>[2x]QYVRIKNWGSGEILHDTLHHKATSDFTCKSKSCLGSIMNPKSLTRGPRDKPTPLEELLPHAIEFINQYYGSFKEAKIEEHLARLEAVTKEIETTGTYQLTLDELIFATKMAWRNAPRCIGRIQWSNLQVFDARNCSTAQEMFQHICRHILYATNNGNIRSAITVFPQRSDGKHDFRLWNSQLIRYAGYQMPDGTIRGDAATLEFTQLCIDLGWKPRYGRFDVLPLVLQADGQDPEVFEIPPD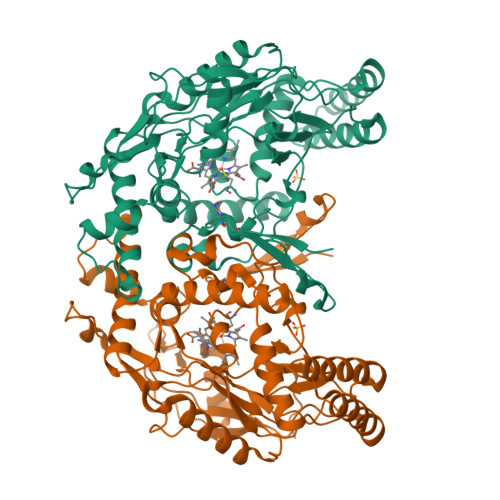LVLEVTMEHPKYEWFQELGLKWYALPAVANMLLEVGGLEFPACPFNGWYMGTEIGVRDFCDTQRYNILEEVGRRMGLETHTLASLWKDRAVTEINVAVLHSFQKQNVTIMDHHTASESFMKHMQNEYRARGGCPADWIWLVPPVSGSITPVFHQEMLNYVLSPFYYYQIEPWKTHIWQ> SNAEAMAALKLVPNNADFAFQFFREVTQEAPNKNIFYSPVSISTAFA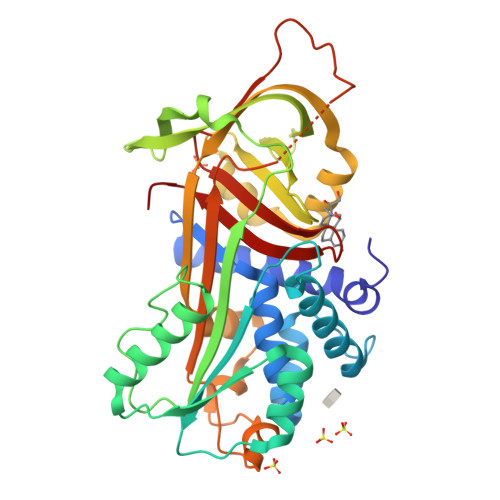MLALGARSATQSQILEGLAFNLTEIQEKEIHEGFHNLIHMLNHPEGGVQLNMMNAIFVTAALALLRKFLDDAKALYQLEAFTTDFNKPTEAEKQINDYIERKTHGKITNLVKDMDPQTVMLLASFVYFKGSWEKPFEAEHTEEREFFVDAETTVKVPMMYQMGRFDFYFDEELSCTVVRLHYNGSATAFLVLPAKGKMKQLEQTLDKETIQKWSDHLFQRFMNLYFPKFSISGSYEISNTLRKMGIVDVFTNQADLSGITGSPDLKVSKVVHKASLDVDEKGTEAAAATAVEIMPISFPPTIEFSHPFLMLIFDRDTNSTLFIGKIVNPTITS>MSTFEDADDEETVTCLQMTIYHPGQQSGIFKSIRFSSKEKFPSIEVVKFGRNSNMCQYTFQDKQVSRIQFVLQPFKQFNSSVLSFEIKNMSKKTSLMVDNQELGY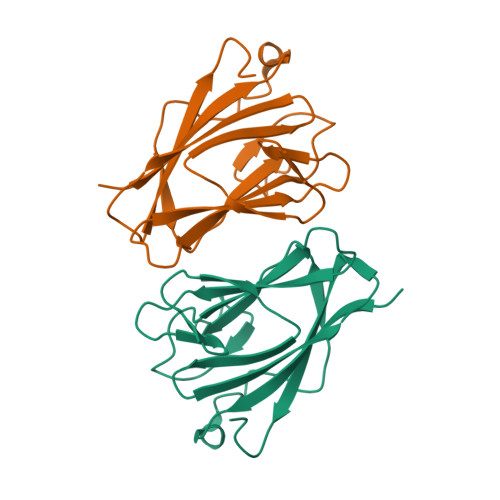LNKMDLPYKCMLRFGEYQFLLQKEDGESVESFETQFIMSSRPLLQENNWPTQNPIPEDGMYSSYFTHRSSPSEMDENELLEHHHHHH[4x]> DLSSLTPGGSMGLQVNRGSQSSLEGAPATAPEPHSLGILHASYSVSHRVRPWWDITSCRQQWTRQILKDVSLYVESGQIMCILGSSGSGKTTLLDAMSGRLGRAGTFLGEVYVNGRALRREQFQDCFSYVLQSDTLLSSLTVRETLHYTALLAIRRGNPGSFQKKVEAVMAELSLSHVADRLIGNYSLGGISTGERRRVSIAAQLLQDPKVMLFDEPTTGLDCMTANQIVVLLVELARRNRIVVLTIHQPRSELFQLFDKIAILSFGELIFCGTPAEMLDFFNDCGYPCPEHSNPFDFYMDLTSVDTQSKEREIETSKRVQMIESAYKKSAICHKTLKNIERMKHLKTLPMVPFKTKDSPGVFSKLGVLLRRVTRNLVRNKLAVITRLLQNLIMGLFLLFFVLRVRSNVLKGAIQDRVGLLYQFVGATPYTGMLNAVNLFPVLRAVSDQESQDGLYQKWQMMLAY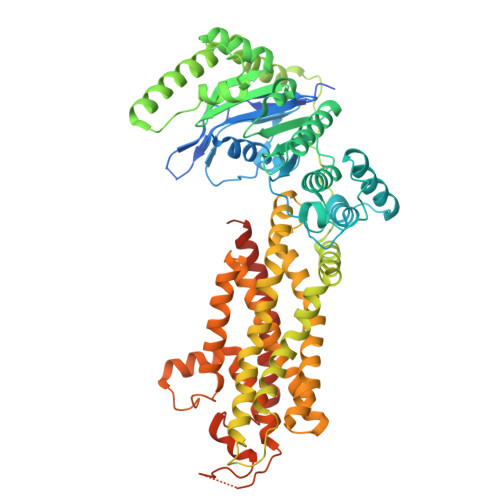ALHVLPFSVVATMIFSSVCYWTLGLHPEVARFGYFSAALLAPHLIGEFLTLVLLGIVQNPNIVNSVVALLSIAGVLVGSGFLRNIQEMPIPFKIISYFTFQKYCSEILVVNEFYGLNFTCGSSNVSVTTNPMCAFTQGIQFIEKTCPGATSRFTMNFLILYSFIPALVILGIVVFKIRDHLISRGSHHHHHHGHHHHHH ethyl 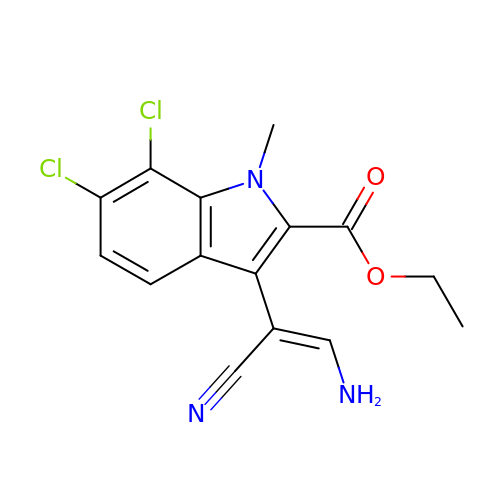3-[(E)-2-amino-1-cyanoethenyl]-6,7-dichloro-1-methyl-1H-indole-2-carboxylate | C15 H13 Cl2 N3 O2 | CXJCGSPAPOTTSF-VURMDHGXSA-N> NLGLEDIIRKAL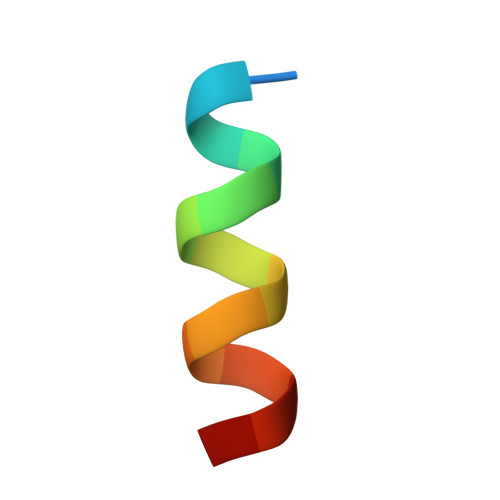MGS> GSHMSAADFEAAVAYVRSLPKEGPVQLDNAAKLQFYSLYKQATEGDVTGSQPWAVQVEARAKWDAWNSCKG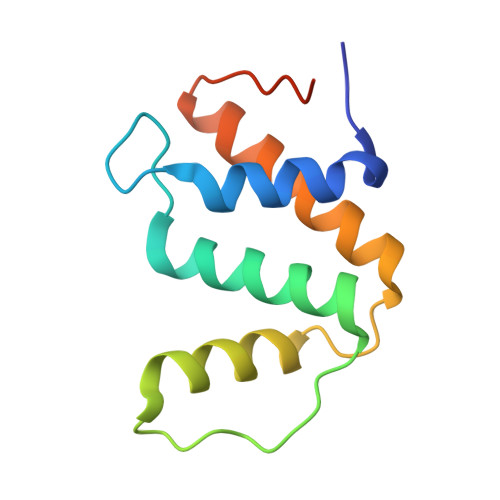MKSEDAKAAYVRRLLTLLRSQGIQWKPGARVQSRL> ATCELALENKSLPGTVHAYVTGHEQGTDRWVLLRPDGSVYRPDSPGAPQTPLPVDCAIPLKGAGAGPVVMTLP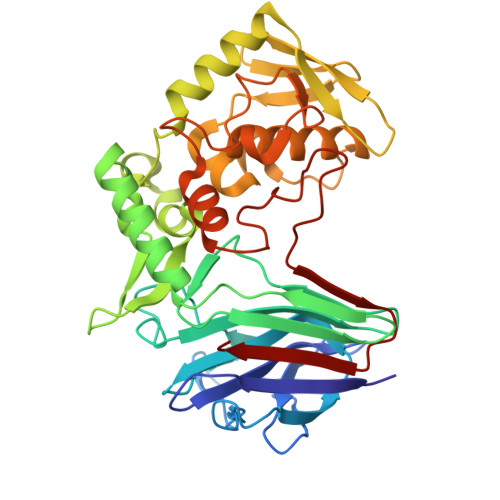QMYGARVYFVRDDKLDFYLNPGPSLVEPAFATPTDPNYGRTWSFCEFTFNPQQLYANISYVDLVTALPIGLTLEGDSTHTVAPLPDGAVQRIADDLTAQAASDGQPWDKLVTRGSDGQVLRVVSPQNLMAPFFDRPDQMPFRDLFTAQIDEVWEKYRSTDLRIDLQGGRGTLAGRVSGDTLTFEGGHTFVKPTSKDIFTCNHGPFANDPADSDDKKALLARIAAGFNRSIMLSHPQQPNGTTVADYYKGGVTNHWSRVVHANSPIGYAFPYDDVRPDGEPDVSGAAHDGNPRRFTVSVGS>[2x]MIVFVRFNSSHGFPVEVDSDTSIFQLKEVVAKRQGVPADQLRVIFAGKELRNDWTVQNCDL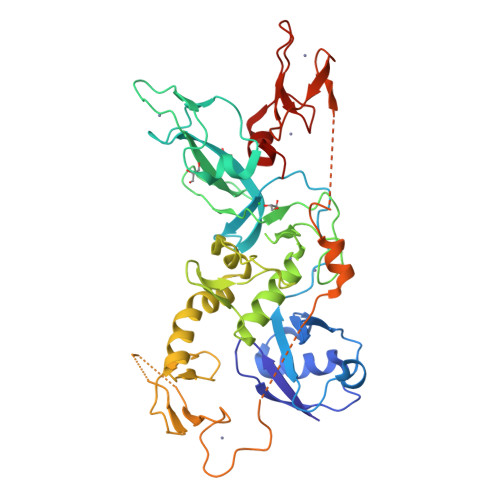DQQSIVHIVQRPWRKGQEMNATNSFYVYCKGPCQRVQPGKLRVQCSTCRQATLTLTQGPSCWDDVLIPNRMSGECQSPHCPGTSAEFFFKCGAHPTSDKETSVALHLIATNSRNITCITCTDVRSPVLVFQCNSRHVICLDCFHLYCVTRLNDRQFVHDPQLGYSLPCVAGCPNSLIKELHHFRILGEEQYNRYQQYGAEECVLQMGGVLCPRPGCGAGLLPEPDQRKVTCEGGNGLGCGFAFCRECKEAYHEGECSAVFEASGTTTQAYRVDERAAEQARWEAASKETIKKTTKPCPRCHVPVEKNGGCMHMKCPQPQCRLEWCWNCGCEWNRVCMGDHWFDV> GSWFFKNLSRKDAERQLLAPGNTHGSFLIRESESTAGSFSLSVRDFDQNQG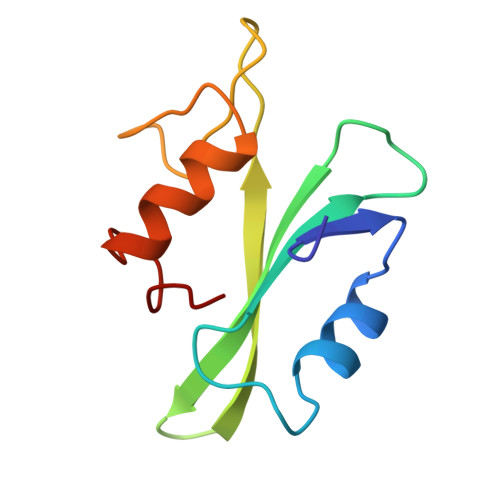EVVKHYKIRNLDNGGFYISPRITFPGLHELVRHYTNASDGLCTRLSR> MAKSYSEQPELHAKAPYRSAMLTYPGNLRQALKDAMADPSKTLMGVAHGIPSTFVTKVLAATKPDFVWIDVEHGMFNRLELHDAIHAAQHHSEGRSLVIVRVPKHDEVSLSTALDAGAAGIVIPHVET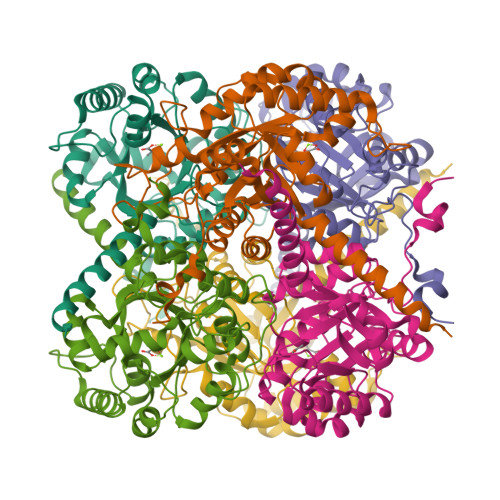VEEVREFVKEMYYGPIGRRSFSPWTFSPGIADASLFPNDPYNVATSNNHVCIIPQIESVKGVENVDAIAAMPEIHGLMFGPGDYMIDAGLDLNGALSGVPHPTFVEAMTKFSTAAQRNGVPIFGGALSVDMVPSLIEQGYRAIAVQFDVWGLSRLVHGSLAQARASAKQFAGQGKAATDGTTDETVDGAAEEVANGVSKVKLDEAGDEDKA> MVKAFWSALQIPELRQRVLFTLLVLAAYRLGAFIPTPGVDLDKIQEFLRTAQGGVFGIINLFSGGNFERFSIFALGIMPYITAAIIMQILVTVVPALEKLSKEGEEGRRIINQYTRIGGIALGAFQGFFLATAFLGAEGGRFLLPGWSPGPFFWFVVVVTQVAGIALLLWMAERITEYGIGNGTSLIIFAGIVVEWLPQILRTIGLIRTGEVNLVAFLFFLAFIVLAFAGMAAVQQA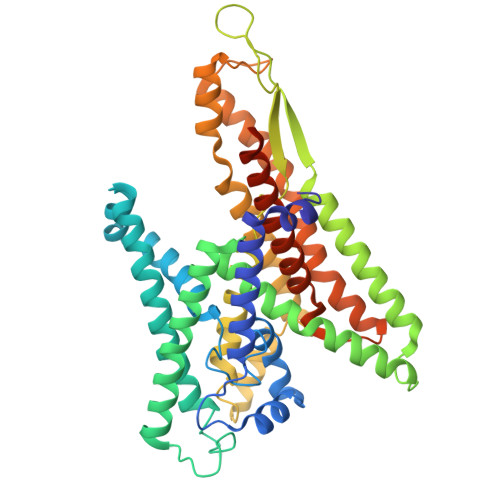ERRIPVQYARGAAGYGGQATYIPIKLNAAGVIPIIFAAAILQIPIFLAAPFQDNPVLQGIANFFNPTRPSGLFIEVLLVILFTYVYTAVQFDPKRIAESLREYGGFIPGIRPGEPTVKFLEHIVSRLTLWGALFLGLVTLLPQIIQNLTGIHSIAFSGIGLLIVVGVALDTLRQVESQLMLRSYEGFLSRGRLRGRNRHHHHHH> TALRQQVETLQGQVQRLQKAFSQYKKVELFPNGRGVGEKIFKT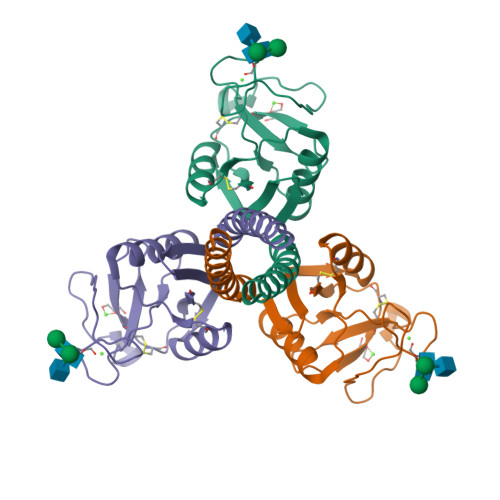GGFEKTFQDAQQVCTQAGGQMASPRSETENEALSQLVTAQNKAAFLSMTDIKTEGNFTYPTGEPLVYANWAPGEPNNNGGSSGAENCVEIFPNGKWNDKACGELRLVICEF>[4x]MHHHHHHSSGRENLYFQG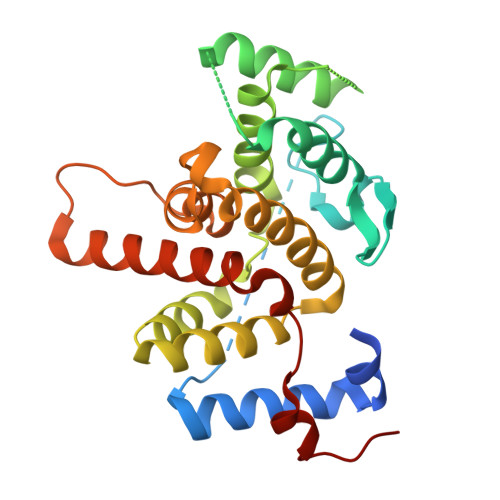MWDQRLVRLALLQHLRAFYGIKVKGVRGQCDRRRHETAATEIGGKIFGVPFNALPHSAVPEYGHIPSFLVDACTSLEDHIHTEGLFRKSGSVIRLKALKNKVDHGEGCLSSAPPCDIAGLLKQFFRELPEPILPADLHEALLKAQQLGTEEKNKATLLLSCLLADHTVHVLRYFFNFLRNVSLRSSENKMDSSNLAVIFAPNLLQTSEGHEKMSSNTEKKLRLQAAVVQTLIDYASDIGRVPDFILEKIPAML In this work, we exhaustively probe the ability of all 36 immobile HJ sequences to form DNA crystals in two different designed systems. Three separate self-assembling DNA crystal systems are described in this report: the “4 × 5” and “4 × 6” designs (collectively referred to as the 4 × N systems), and a third construct with a “scrambled” sequence variant of the 4 × 6 lattices. Self-assembly was mediated by three constituent oligonucleotides: (S1) containing four sequence repeats of either 5 or 6 bases; (S2) composed of 21 bases containing complementary regions to both (S1); and (S3) which forms the second junction crossover. The HJ serves as the fundamental component at the core of each unit, and the ultimate assembly of the full lattice is facilitated by the complementary 2-base sticky ends that tail each duplex.

Because the 4 × 6 system yielded R3 symmetry in 5 of 17 junctions, we considered whether the downstream sequences adjacent to the junction could play a role in crystallization efficiency, junction angle, and symmetry preference, or if the HJ alone was the singular determinant. To investigate this possibility, we designed “scrambled” sequences with targeted base substitutions, while maintaining GC content, along each “stem”. Contrary to the buffer preference observed with the native P32 crystals, the scrambled systems exhibited an exclusive preference towards low salt buffers, much like the native R3 crystals. Remarkably, only J1 and J2 retained the P32 symmetry, with all others yielding an R3 lattice. There appeared to be only a marginal difference in the average cell lengths in the R3 scramble crystals (a = b = 113.04 c = 51.10) relative to the native 4 × 6 sequences: the a, b axis trended ~2 Å shorter and c ~1.3 Å longer, whereas in the J1 and J2 cases, the crystals were in good agreement with the original 4 × 6 motif. The average angles of the R3 and P32 crystals were 61.00° (σ = 1.21) and 58.05° (σ = 1.39), respectively. Further, we observed modest improvements in resolution, reaching as high as 2.7 Å in J36. Notably, all junctions preventing crystallization compared to its original counterpart remained fatal and all relative cavity dimensions and volumes remained unperturbed. However, in the majority of the crystal structures reported here, the cacodylate anion indeed fits best into the electron density map of our X-ray structures, due to the presence of sodium cacodylate in the crystallization solution. A complete description of the comprehensive, experimental evidence for this arsenic has been described in our previous work. This seemingly counterintuitive result can be rationalized in several ways: First, the cacodylate could be stabilized at this site by hydrogen bonding and interactions with the solvent, both of which are known to provide stabilization for anionic binding even at regions with negative surface potentials.

> GAACGACACAGA;> CGTCGACTC;> TCTACG;> TCGAGTCGGTGTCGT> MVFPSSVYVPDEWEVSREKITLLRELGQGSFGMVYEGNARDIIKGEAETRVAVKTVNESASLRERIEFLNEASVMKG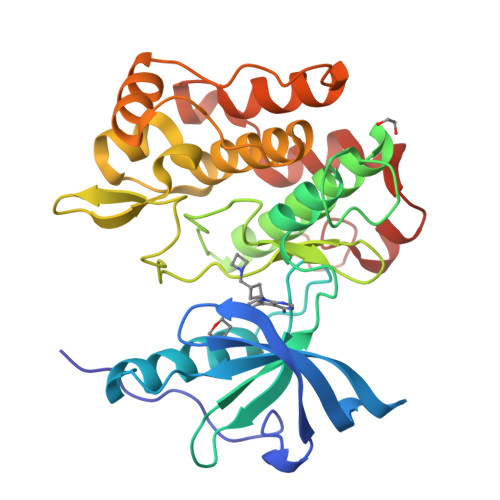FTCHHVVRLLGVVSKGQPTLVVMELMAHGDLKSYLRSLRPEAENNPGRPPPTLQEMIQMAAEIADGMAYLNAKKFVHRNLAARNCMVAHDFTVKIGDFGMTRDIYETDYYRKGGKGLLPVRWMAPESLKDGVFTTSSDMWSFGVVLWEITSLAEQPYQGLSNEQVLKFVMDGGYLDQPDNCPERVTDLMRMCWQFNPKMRPTFLEIVNLLKDDLHPSFPEVSFFHSEENK N-(3,5-dichlorobenzyl)-N'-(1H-imidazo[4,5-b]pyridin-2-yl)propane-1,3-diamine | C16 H17 Cl2 N5 | 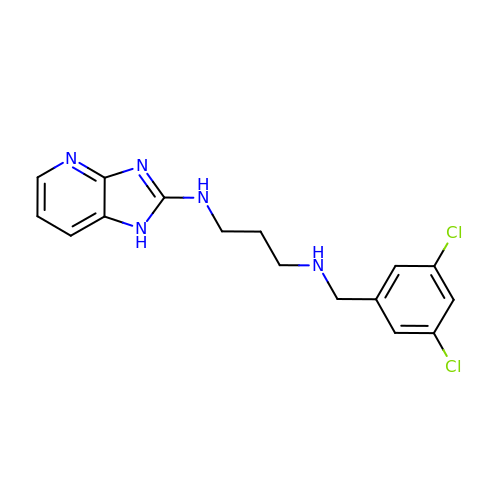JOBYCWUVGFAKEK-UHFFFAOYSA-N N-[(1R,2s,3S,5s,7s)-5-hydroxytricyclo[3.3.1.1~3,7~]dec-2-yl]-5,7-dimethylpyrazolo[1,5-a]pyrimidine-3-carboxamide | C19 H24 N4 O2 | 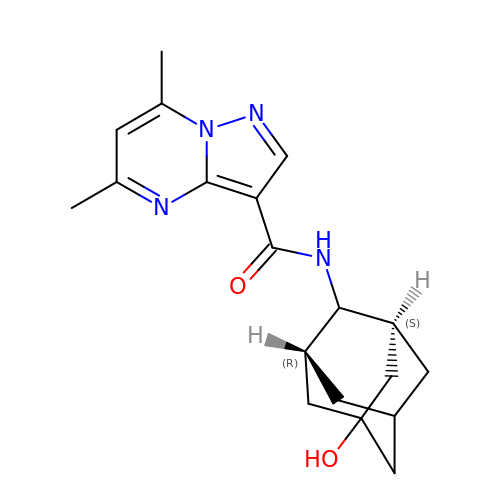XAKHQMQFIBQWBI-VTPCDMJMSA-N> LWPWPQNFQTSDQRYVLYPNNFQFQYDVSSAAQPGCSVLDEAFQRYRDLLFGSGSWPRPYLTGKRHTLEKNVLVVSVVTPGCNQLPTLESVENYTLTINDDQCLLLSETVWGALRGLETFSQLVWKSAEGTFFINKTEIEDFPRFPHRGLLLDTSRHYLPLSSILDTLD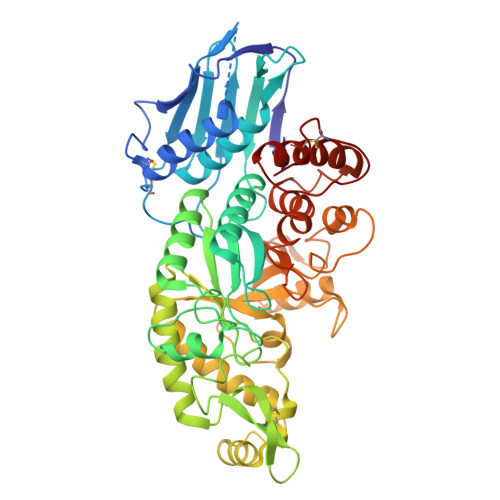VMAYNKLNVFHWHLVDDPSFPYESFTFPELMRKGSYNPVTHIYTAQDVKEVIEYARLRGIRVLAEFDTPGHTLSWGPGIPGLLTPCYSGSEPSGTFGPVNPSLNNTYEFMSTFFLEVSSVFPDFYLHLGGDEVDFTCWKSNPEIQDFMRKKGFGEDFKQLESFYIQTLLDIVSSYGKGYVVWQEVFDNKVKIQPDTIIQVWREDIPVNYMKELELVTKAGFRALLSAPWYLNRISYGPDWKDFYVVEPLAFEGTPEQKALVIGGEACMWGEYVDNTNLVPRLWPRAGAVAERLWSNKLTSDLTFAYERLSHFRCELLRRGVQAQPLNVGFCEQEFEQT> QTEDYCL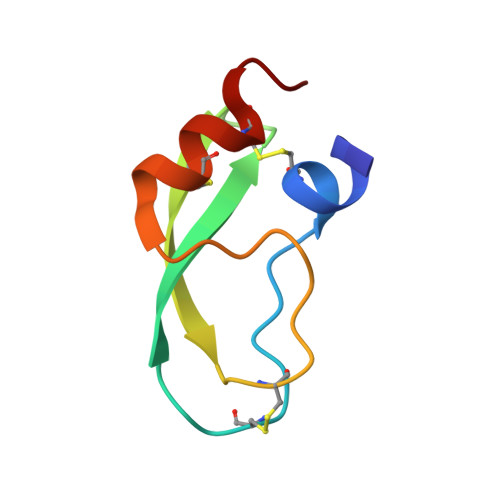ASNKVGRCRGSFPRWYYDPTEQICKSFVYGGCLGNKNNYLREEECILACRGVQ> QFHVKSGLQIKKNAIIDDYKVTSQVLGLGINGKVLQIFNKRTQEKFALKMLQDCPKARREVELHWRASQCPHIVRIVDVYENLYAGRKCLLIVMECLDGGELFSRIQDRGDQAFTEREASEIMKSIGEAIQYLHSINIAHRDVKPENLLYTSKRPNAILKLTDFGFAKETTSHNSLTTPCYTPYYVAPEVLGPEKYDKSCDMWSLGVIMYILLCGYPPFYSNHGLAISPGMKTRIRMGQYEFPNPEWSEVSEEVKMLIRNLLKTEPTQRMTITEFMNHPWIMQST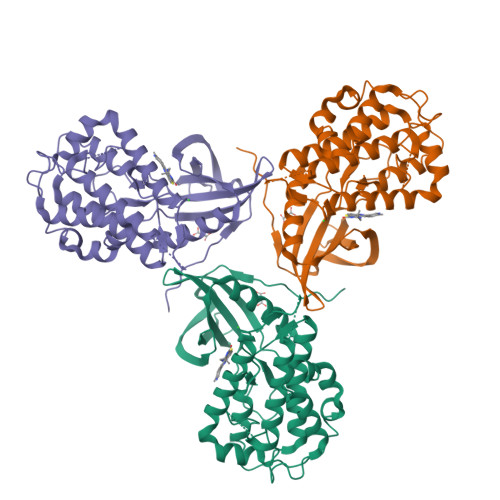KVPQTPLHTSRVLKEDKERWEDVKEEMTSALATMRVDYEQIK> MSMLKREDWYDLTRTTNWTPKYVTENELFPEEMSGARGISMEAWEKYDEPYKITYPEYVSIQREKDSGAYSIKAALERDGFVDRADPGWVSTMQLHFGAIALEEYAASTAEARMARFAKAPGNRNMATFGMMDENRHGQIQLYFPYANVKRSRKWDWAHKAIHTNEWAAIAARSFFDDMMMTRDSVAVSIMLTFAFETGFSNMQFLGLAADAAEAGDHTFASLISSIQTDESRHAQQGGPSLKILVENGKKDEAQQMVDVAIWRSWKLFSVLTGPEMDYYTPLESRNQSFKEFMLEWI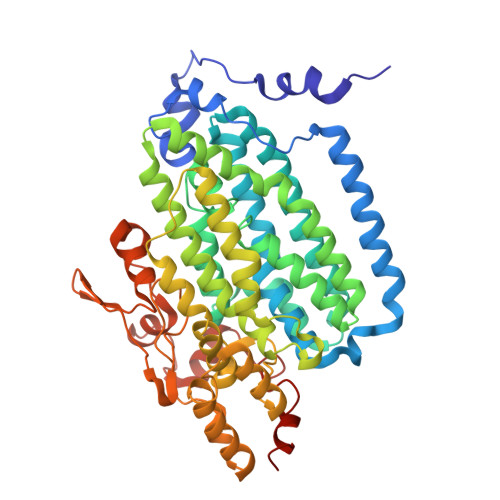VAQFERQLLDLGLDKPWYWDQFMQDLDETHHGMHLGVWYWRPTVWWDPAAGVSPEEREWLEEKYPGWNDTWGQCWDVITDNLVNGKPELTVPETLPTICNMCNLPIAHTPGNKWNVKDYQLEYEGRLYHFGSEADRWCFQIDPERYKNHTNLVDRFLKGEIQPADLAGALMYMSLEPGVMGDDAHDYEWVKAYQKKTNAA>ATATAATPAAEATSRGWNDYSCKPSAAHPRPVVL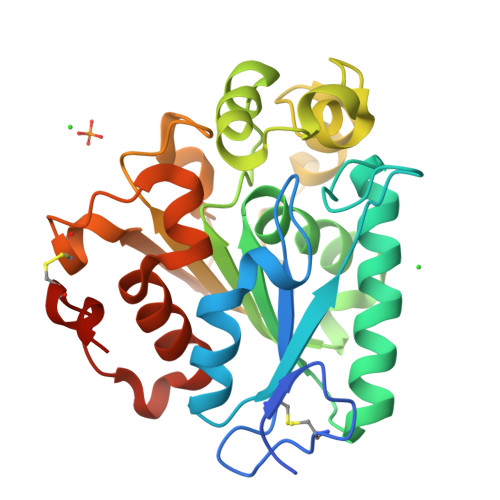VHGTFGNSIDNWLVLAPYLVNRGYCVFSLDYGQLPGVPFFHGLGPIDKSAEQLDVFVDKVLDATGAPKADLVGHSQGGMMPNYYLKFLGGADKVNALVGIAPDNHGTTLLGLTKLLPFFPGVEKFISDNTPGLADQVAGSPFITKLTAGGDTVPGVRYTVIATKYDQVVTPYRTQYLDGPNVRNVLLQDLCPVDLSEHVAIGTIDRIAFHEVANALDPARATPTTCASVIGHHHHHH[3x]>GSSVYRIPLADMTFWSWMSYLKELPDIDESRNPILKRLLSGSFLRRDGSTTVNVRVPARELVRLLSLTPEQQREGVSAKVRLINLLDPKYSVYEPYLYREILPKRSPLLLPSLGEYRGAFLTYIFHPLSKGLVGDMLETGRSHPDVQVLAANMVAALKSLHNLGLLHRSIELNSFSVLPDGTVVLGGLDTAAPIGTETRLWVGFFGQETAPEIDRNFLADLALTQGRHTVKSDVYSLGVAFRNLVQLLGNGNLGPEDRGAVRQDHLELLDKLSQKMIEEEPGNRPTIEEIMKDPLFEGLNFEDIEEGKARPFRY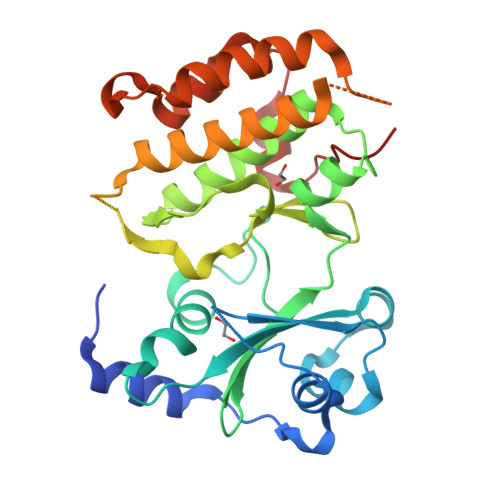KQNRL[6x]>AMADLEQKVLEMEASTYDGVFIWKISDFPRKRQEAVAGRIPAIFSPAFYTSRYGYKMCLRIYLNGDGTGRGTHLSLFFVVMKGPN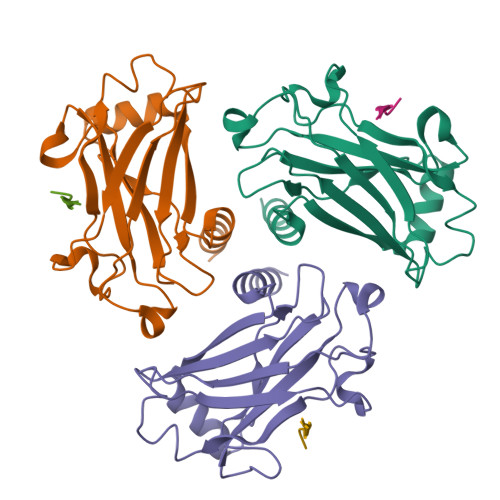DALLRWPFNQKVTLMLLDQNNREHVIDAFRPDVTSSSFQRPVNDMNIASGCPLFCPVSKMEAKNSYVRDDAIFIKAIVDLTGL[6x];>[6x]XPIQEE(3S)-3-benzyl-5-[9-ethyl-8-(2-methylpyrimidin-5-yl)-9H-purin-6-yl]-3-methyl-1,3-dihydro-2H-indol-2-one | C28 H25 N7 O | 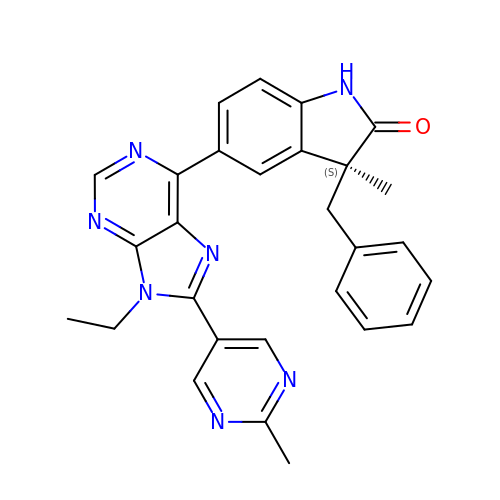FFRRAJYYORCXFZ-NDEPHWFRSA-N> AHHHHHHGSMLKEVHELLNRIWGDIFELREELKEELKGFTVEEVSEVFNAYLY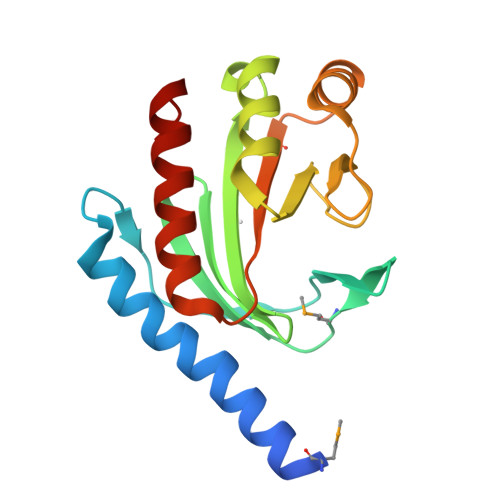IDGKWEEMKYPHPAFAVKPGGEVGATPQGFYFVFAFPKEELSKEFIEDVIRAFEKLFIYGAENFLEDFYNFEHPISGDEVWDRIVNSDEEMINFEVDLGFDKEEVKREIKRFIELARRYNLL Bacterial genomes usually encode two type IIA enzymes, topo IV and DNA gyrase, each composed of two subunits (ParC and ParE in topo IV, GyrA and GyrB in gyrase) assembled into a functional heterotetramer i.e. C2E2 and A2B2, respectively. Both enzymes act by passing a duplex DNA segment through a transient double-stranded DNA break in another helical region. By contrast, topo IV is a decatenating enzyme that resolves interlinked daughter chromosomes following DNA replication. For example, though gyrase is the universal target of quinolones in gram-negative bacteria, topo IV is the primary (or dual) target of many quinolones in gram-positive pathogens such as Streptococcus pneumoniae, a major cause of pneumonia and other serious infections.

To gain insight into the mechanism of S. pneumoniae topo IV and its interaction with DNA and quinolones, the structure of the ParC55 fragment has been solved and the model was refined to R = 22.30% (R-free = 27.55%) at 2.7 Å resolution using wild-type ParC55 data (twinning fraction = 0.323, twinning operator = (k,-h,l)). ParC55 forms a biological dimer in a ‘closed’ conformation in this crystal form generating a ring-like structure with outer dimensions of 100×100×50 Å and with a central hole approximately 30 Å in diameter, which is wide enough to pass a duplex DNA. Each monomer of ParC55 contains two distinct regions labeled ‘head’ and ‘tail’ and exhibits an overall structural fold similar to the one observed for other topoisomerases. The N-terminal proximal head contains the CAP-like (catabolite gene activator protein) DNA-binding domain and the ‘tower’. The CAP-like domain is composed of a helix-turn-helix structural motif (helices α3 and α4) typical for DNA-binding proteins, with the active site Arg 117 and Tyr 118 on the neighboring ‘100-122’ loop. The residues Ser 79 and Asp 83, which upon mutation give rise to quinolone-resistant pneumococci, are located primarily within the helix α4 in close proximity to the active-site tyrosine and are oriented towards the predicted position of the bound DNA. In the closed conformation, the ParC55 monomers form a tight contact between the α3 helices with a mean center-to-center distance of 10 Å resulting in the protein-protein interface with a buried surface area of 706 Å2. In the ‘closed’ S. pneumoniae ParC structure, the loop is positioned vertically and stands on the side of the DNA-binding groove orienting the active-site tyrosine towards the expected position of the DNA backbone and exposing the active-site helices (α3 and α4) to the predicted protein-DNA interface. S. pneumoniae ParC55 folds into a similar closed conformation to that of E. coli GyrA However, interestingly, the DNA binding site formed by the pneumococcal ParC55 dimer differs markedly in its electrostatic charge distribution from both the E. coli ParC and GyrA dimers.

>MSNIQNMSLEDIMGERFGRYSKYIIQDRALPDIRDGLKPVQRRILYSMNKDSNTFDKSYRKSAKSVGNIMGNFHPHGDSSIYDAMVRMSQNWKNREILVEMHGNNGSMDGDPPAAMRYTEARLSEIAGYLLQDIEKKTVPFAWNFDDTEKEPTVLPAAFPNLLVNGSTGISAGYATDIPPHNLAEVIDAAVYMIDHPTAKIDKLMEFLPGPDFPTGAIIQGRDEIKKAYETGKGRVVVRSKTEIEKLKGGKEQIVITEIPYEINKANLVKKIDDVRVNNKVAGIAEVRDESDRDGLRIAIELKKDANTELVLNYLFKYTDLQINYNFNMVAIDNFTPRQVGIVPILSSYIAHRREVILARSRFDKEKAEKRLHIVEGLIRVISILDEVIALIRASENKADAKENLKVSYDFTEEQAEAIVTLQLYRLTNTDVVVLQEEEAELREKIAMLAAIIGDERTMYNLMKKELREVKKKFATPRLSSLEDTAKALEHHHHHH[4x]>MAGTDKRKQSLYFPEEMLKEIQEEATRQDRSLSWVVQQAWKIARERIKSFPAVNDVTGDERQDP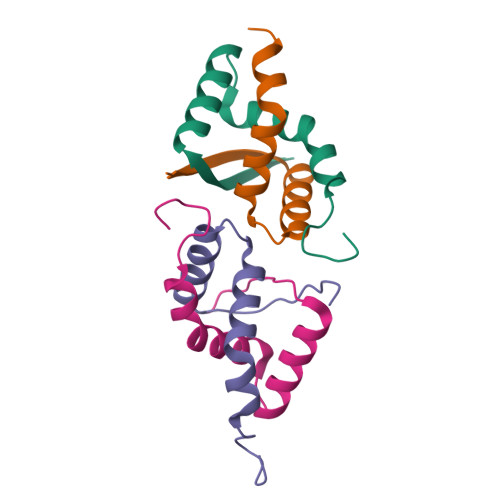REE[3x]3-CARBOXAMIDO-1,3,5(10)-ESTRATRIEN-17(R)-SPIRO-2'(5',5'-DIMETHYL-6'OXO)TETRAHYDROPYRAN | C25 H33 N O3 | 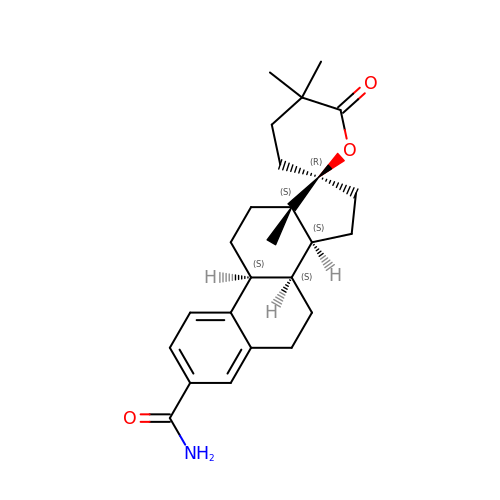YVAJWBACBRSVPR-NDUHRLLKSA-N>[2x]GAMAQRMVWVDLEMTGLDIEKDQIIEMACLITDSDLNILAEGPNLIIKQPDELLDSMSDW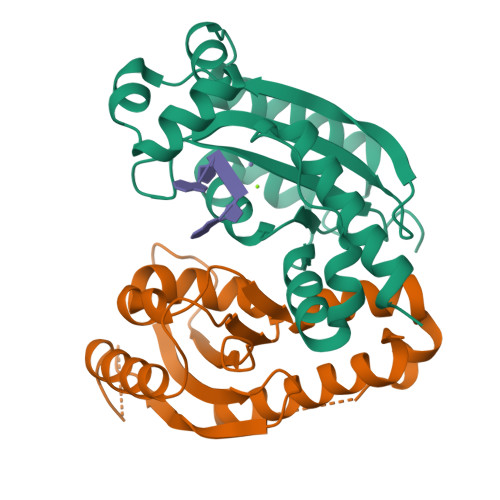CKEHHGKSGLTKAVKESTITLQQAEYEFLSFVRQQTPPGLCPLAGNSVHEDKKFLDKYMPQFMKHLHYRIIDVSTVKELCRRWYPEEYEFAPKKAASHRALDAISESIKELQFYRNNIFK> M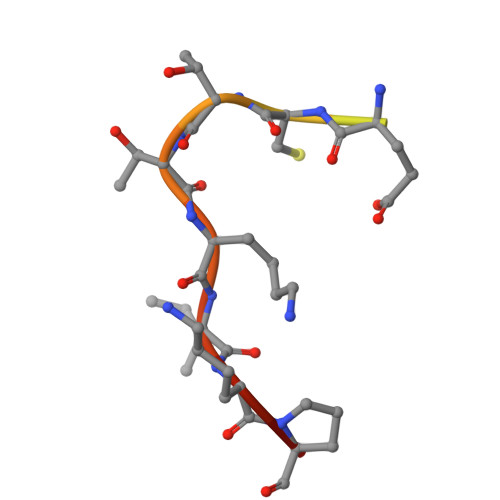DDDDKMDNECTTKIKPR> MTVTAPNALNFECETGNYHTFCPISCVAWLYQKIEDSFFLVIGTKTCGYFLQNAMGVMIFAEPRYAMAELEEGDISAQLNDYEELKRLCLEIKRDRNPSVIVWIGTCTTEIIKMDLEGLAPKLEAEIGIPIVVARANGLDYAFTQGEDTVLAAMAARCPTSTAISDPEERNPIQRLLNFGKKKEEVQAQSSQYHPHPPLVLFGSLPDPVVTQLTLELKKQGIKVSGWLPAKRYTELPVIDEGYYVAGVNPFLSRTATTLIRRRKCQLIT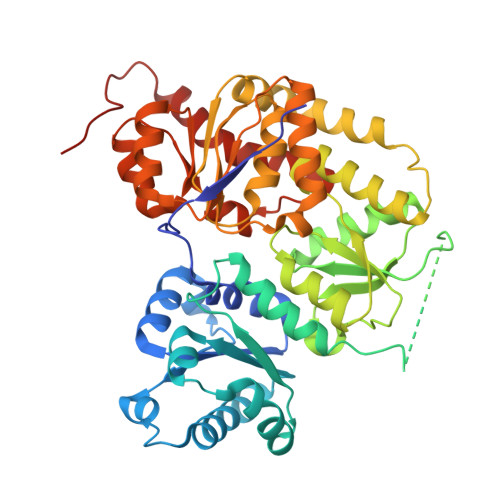APFPIGPDGTRTWIEQICATFGIQPQGLAEREAETWQKLSDYLELVRGKSVFFMGDNLLEISLARFLIRCGMRVLEIGIPYMDKRYQAAELALLSQTCAEMGHPLPTIVEKPDNYNQLQRIKALQPDLVITGMAHANPLEARGISTKWSVEFTFAQIHGFGNARDILELVTRPLRRNQALAGLGWQKLVAH propyl 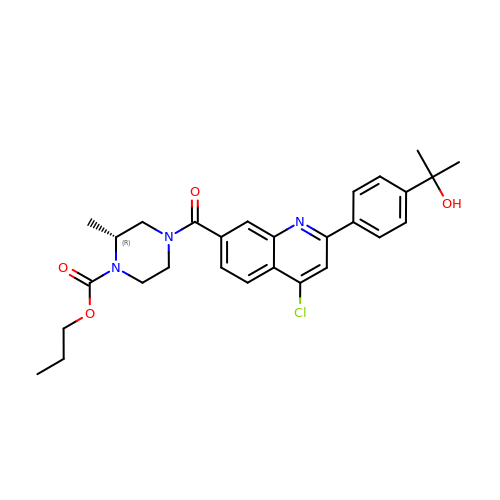(2~{R})-4-[4-chloranyl-2-[4-(2-oxidanylpropan-2-yl)phenyl]quinolin-7-yl]carbonyl-2-methyl-piperazine-1-carboxylate | C28 H32 Cl N3 O4 | BURBRCSDCXUEJO-GOSISDBHSA-N>[2x]MGSSHHHHHHSSGLVPRGSHSQPSTANGGFPSVVVTAVTATTSISPDIESTWKGLLAGESGIHALEDEFVTKWDLAVKIGGHLKDPVDSHMGRLDMRRMSYVQRMGKLLGGQLWESAGSPEVDPDRFAVVVGTGLGGAERIVESYDLMNAGGPRKVSPLAVQMIMPNGAAAVIGLQLGARAGVMTPVSACSSGSEAIAHAWRQIVMGDADVAVC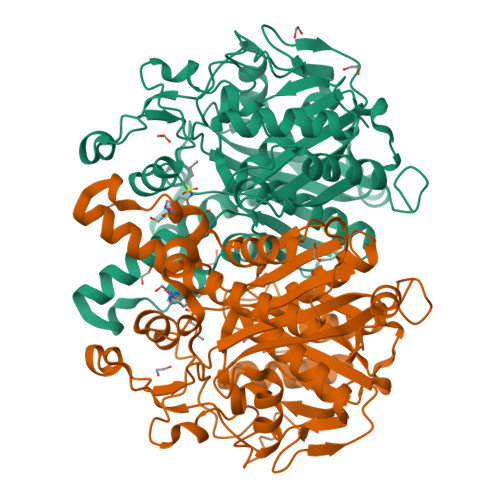GGVEGPIEALPIAAFSMMRAMSTRNDEPERASRPFDKDRDGFVFGEAGALMLIETEEHAKARGAKPLARLLGAGITSDAFHMVAPAADGVRAGRAMTRSLELAGLSPADIDHVNAHGTATPIGDAAEANAIRVAGCDQAAVYAPKSALGHSIGAVGALESVLTVLTLRDGVIPPTLNYETPDPEIDLDVVAGEPRYGDYRYAVNNSFGFGGHNVALAFGRY> C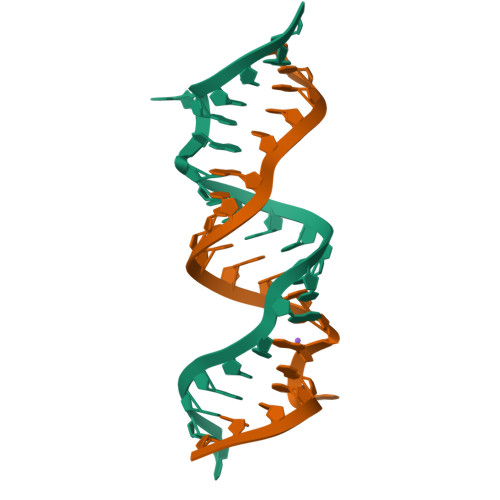GCGUCACCCCGGGCAAGUCGC;> GCGUCACCCCGGGCAAGUCGC>SNAMDTLQFQKNPETAAKMSAYMKHQFVFAGIPAPERQALSKQLLKESHTWPKEKLCQEIEAYYQKTEREYQYVAIDLALQNVQRFSLEEVVAFKAYVPQKAWWDSVDAWRKFFGSWVALHLTELPTI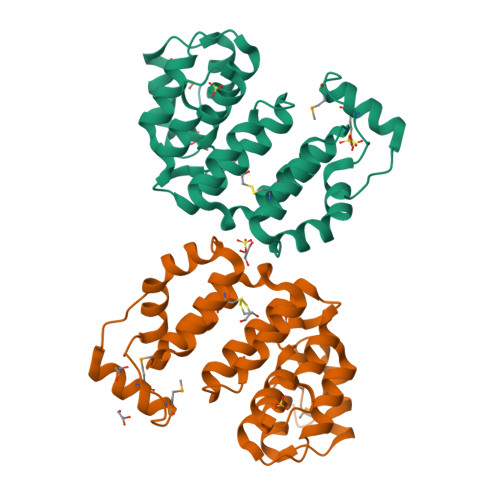FALFYGAENFWNRRVALNLQLMLKEKTNQDLLKKAIIYDRTTEEFFIQKAIGWSLRQYSKTNPQWVEELMKELVLSPLAQREGSKYLAKASE[2x]>MSVLISGASGYIAKHIVRVLLEQNYKVIGTVRSQDKADKLLKQYNNPNLSYEIVPEIANLDAFDDIFKKHGKEIKYVIHAASPVNFGAKDLEKDLVIPAINGTKNMFEAIKKYAPDTVERVVMTASYASIMTPHRQNDPTLTLDEETWNPVTEENAYENVFTAYCASKTFAEKEAWKFVKENSDAVKFKLTTIHPSFVFGPQNFDEDVTKKLNVSCEIINGLLHAPFDTKVEKTHFSQFIDVRDVAKTHVLGFQKDELINQRLLLCNGAFSQQDIVNVFNEDFPELKGQFPPED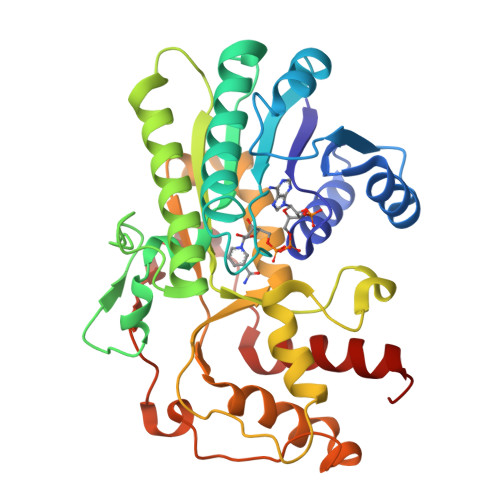KDTDLNKGVTGCKIDNEKTKKLLAFEFTPFHKTIHDTVYQILHKEGRV[2x]> FSQQIYGVVYGNVTFHVPSNVPLKEVLWKKQKDKVAELENSEFRAFSSFKNRVYLDTVSGSLTIYNLTSSDEDEYEMESPNITDT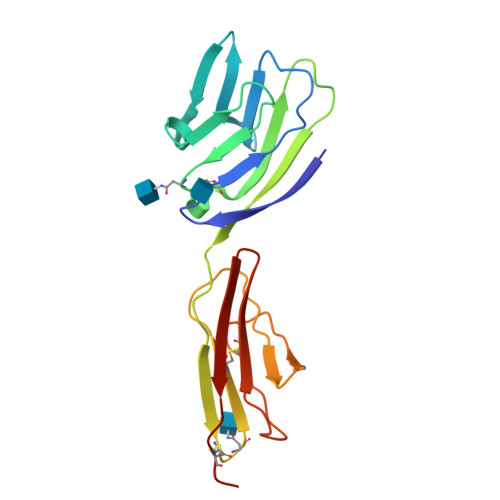MKFFLYVLEMVSKPMIYWECSNATLTCEVLEGTDVELKLYQGKEHLRSLRQKTMSYQWTNLRAPFKCKAVNRVSQESEMEVVNCPE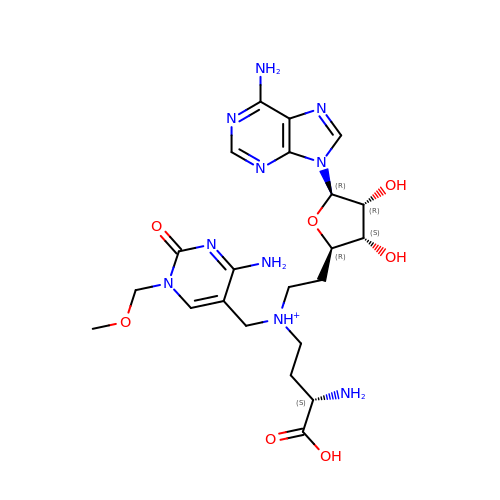2-[(2~{R},3~{S},4~{R},5~{R})-5-(6-aminopurin-9-yl)-3,4-bis(oxidanyl)oxolan-2-yl]ethyl-[[4-azanyl-1-(methoxymethyl)-2-oxidanylidene-pyrimidin-5-yl]methyl]-[(3~{S})-3-azanyl-4-oxidanyl-4-oxidanylidene-butyl]azanium | C22 H33 N10 O7 | GZMYJIXALPWXCM-WUMBASEESA-O> IPCGESCVWIPCISSAIGCSCKSKVCYRNG;> IPCGESCVWLPCISSAIGCSC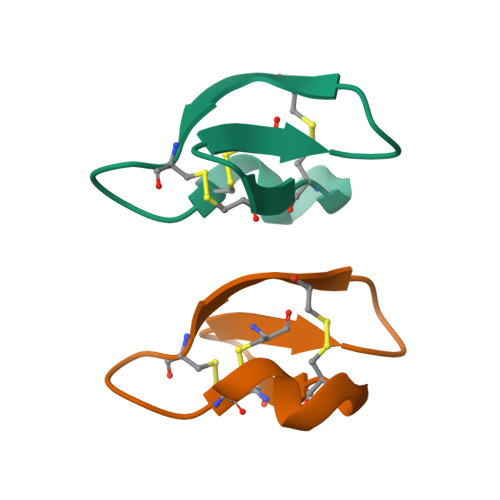KSKVCYRNG> MLTEGISIQSYDGHTFGALVGSPAKAPAPVIVIAQDIFGVNAFMRETVSWLVDQGYAAVCPDLYARQAPGTALDPQDERQREQAYKLWQAFDMEAGVGDLEAAIRYARHQPYSNGKVGLVGYSLGGALAFLVASKGYVDRAVGYYGVGLEKQLNKVPEVKHPALFHMGGQDH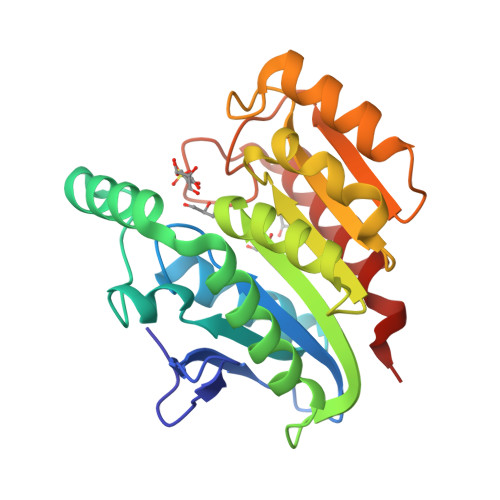FVPAPSRQLITEGFGANPLLQVHWYEEAGHSFARTGSSGYVASAAALANERTLDFLVPLQSRKP>[4x]RIVVYGGTLQYFRVPRNSWERMLKKMKSHGLNTIDTYIAWNWHEPQEGLFDFTGETHPQRDLVGFLDLAQKLGFYVIIRPGPYICGEWKNGGIPEWLINSHPEILAKGPNGTLPRDIYYPPITYLHPTYLEYVMKWYENVFPIIKEYLYSNGGPIINVTIDDEPSYWETIF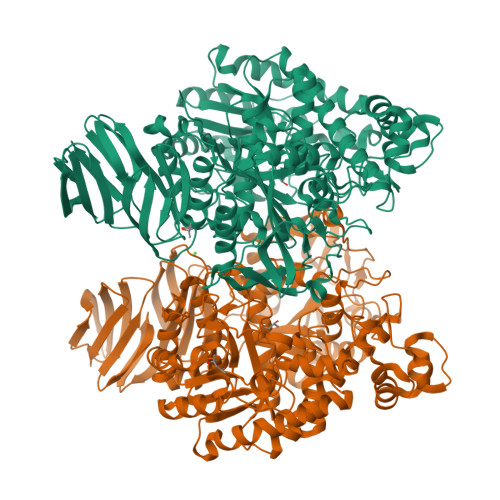QAFLTDYNEIVVKENGIWHSWLKENYQLDELEERYGQKFSDYAEIVPPTSFSEPLPKILDWHHFKIWMINEYVRILYEKIKKYVDVPISILDPYLLLAAWKEFYLYVTKHKLDIHLWTEFWYSFYRTFDFKEDRLGHLYYKTGVYRYYINKLKTPPLSIETQTSLANVIEKDEAELLYALLPALGIHNINYYLYVGGENPKGYESHNGATWDVYSPIGLDGRERQHVEPIKWIGEFLKSNMDFIESQLKPKVAFGMYEPYEALSMWGHRPESFEESVNLQEYLFGERGLLTLLAMSNVPFDVIDLELSTVEEMLQYEQIWIYSLDFMSREVQEKLARYVEEGGNLVILPTLPSLDENMKPYTKLRDFLGIEVEKAKARDNMRLIPYISVDAEEIDRMVVRNVVREVKGGKAIAWVGDKVVGVMVRKGKGSAVVLGFRLQYYSSYHDLHRKFVDKILQLQGIERDFEVSNRDIIVIPRGNYLVVVNPRDDKVTGKVRYRGVEFNVELNKRGVLYIPINVEINGIKVLYATATPVGRGEGTIRFRNHLANVTEIAINGKIKEVSGGYILQEKSSGEKNIYVIKHESETFEIRV>[2x]GAMPHDPSFTPTQLAARAAYLLRGNDLGTMTTAAP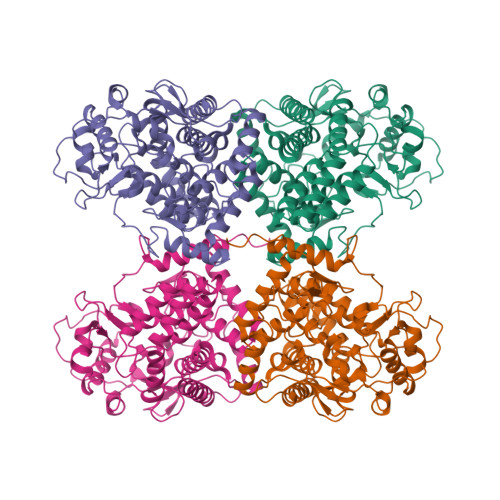LLYPHMWSWDAAFVAIGLAPLSVERAVVELDTLLSAQWRNGMIPHIVFANGVDGYFPGPARWATATLADNAPRNRLTSGITQPPVHAIAVQRILEHARTRGRSTRAVAEAFLDRRWGDLMRWHRWLAECRDRNERGRITLYHGWESGMDNSPRWDSAYANVVPGKLPEYQRADNVIITDPSQRPSDGEYDRYLWLLEEMKAVRYDDERLPSVMSFQVEDVFFSAIFSVACQVLAEIGEDYKRPHADVKDLYLWAERFRAGVVETTDQRTGAARDFDVLAEKWLVTETAAQFAPLLCGGLPHDRERALLKLLEGPRFCGHPDLKYGLIPSTSPVSRDFRPREYWRGPVWPVLTWLFSWCFARRGWAERARLLRQEGLRQASDGSFAEYYEPFTGEPLGSMQQSWTAAAVLDWLG The events that dictate whether the HRSV RdRp either transcribes or replicates are unclear, although the components of a replicating RdRp and a transcribing RdRp are different; the replicase requires the phosphoprotein (P), along with the large catalytic component (L), whereas the transcriptase additionally requires the M2-1 protein. M2-1 is 194 amino acids in length, binds zinc atoms, and exists in solution as a tetramer. Of these, the best-characterized role is that of a transcription factor, in which M2-1 is thought to enhance polymerase processivity by suppressing transcription termination both intragenically and intergenically. In addition, M2-1 interacts with both viral RNA and P. This ability of M2-1 to interact with RNA and P is required for productive transcription, and each monomer within the tetramer can potentially interact with both an RNA molecule and P at an overlapping binding site, suggesting that binding of these ligands at each binding site is mutually exclusive.

We present the crystal structure of M2-1 in complex with the P interaction domain, at a resolution of 2.4 Å, which defines the orientation of the M2-1 and P moieties in the heteromultimeric complex. The electron density difference maps revealed a continuous area of density not accounted for by M2-1 and which appeared to be a peptide that exhibited helical secondary structure. On the basis of this model, we propose that, in the absence of RNA, each M2-1 tetramer associates with a single P tetramer, with all four P binding sites of M2-1 being occupied. The M2-1/P interface includes ionic, hydrophobic, and hydrogen bond interactions, and the critical contribution of these contacts to complex formation was assessed using a minigenome assay. There is a total of 10 plausible hydrogen bonds, with R126 making what appear to be important salt bridges to E104 and E107. There are a multitude of hydrophobic interactions along the length of the P peptide, highlighted by L148 of M2-1 packing against L101 and Y102 of the P peptide. The root mean square deviation (RMSD) on superposition of 158 carbon alphas is only 1.097 Å, suggesting very little structural rearrangement on P binding. The M2-1 side chains of R126 and Y134 move to satisfy the hydrogen bonds, as described in Fig. 3, but other than that, there is little movement of side chains required to accommodate the P peptide. The loop on M2-1 containing S58 and S61 (19), which are dynamically phosphorylated in HRSV-infected cells, appears to be slightly more ordered (the electron density for this region is clearer) in the complex crystal structure. The simultaneous incorporation of altered M2-1 and P proteins had an additive effect on minigenome activity, with most reduced activity exhibited by combining mutants R126E and F98A, which reduced eGFP expression to that of the minus M2-1 control.

>MSRRNPCKFEIRGHCLNGKRCHFSHNYFEWPPHALLVRQNFMLNRILKSMDKSIDTLSEISGAAELDRTEEYALGVVGVLESYIGSINNITKQSACVAMSKLLTELNSDDIKKLRDNEELNSPKIRVYNTVISYIESNRKNNKQTIHLLKRLPADVLKKTIKNTLDIHKSITINNPKESTVSDTNDHAKNNDTT[4x];>[4x]DPTPSDNPFSKLYKETIETFD> AQTVPYGIPLIKADKVQ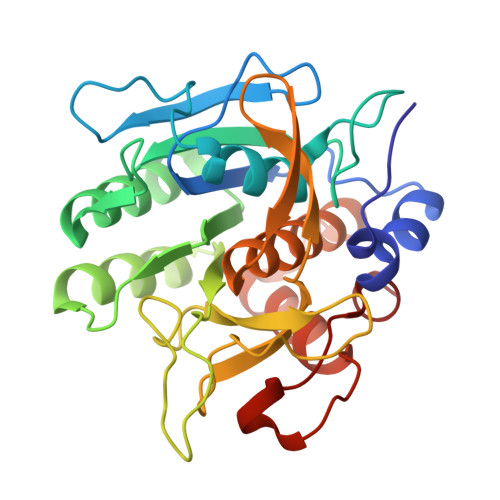AQGFKGANVKVAVLDTGIQASHPDLNVVGGASFVAGEAYNTDGNGHGTHVAGTVAALDNTTGVLGVAPSVSLYAVKVLNSSGSGSYSGIVSGIEWATTNGMDVINMSLGGASGSTAMKQAVDNAYARGVVVVAAAGNSGNSGSTNTIGYPAKYDSVIAVGAVDSNSNRASFSSVGAELEVMAPGAGVYSTYPTNTYATLNGTSMASPHVAGAAALILSKHPNLSASQVRNRLSSTATYLGSSFYYGKGLINVEAAAQ> MSYSAYFAKAGFQFPAGLSALVAGIVALNVCTG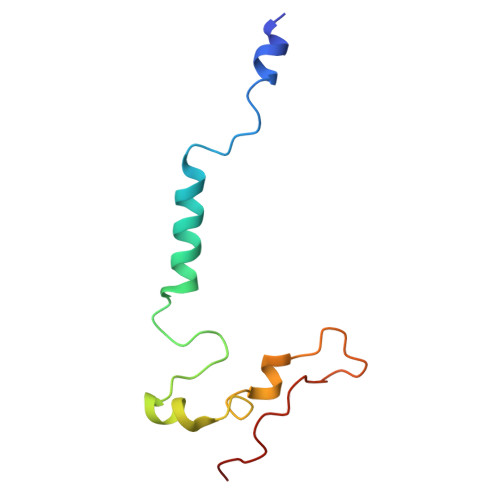RPTKGTKEISNAEYNATPIGYLQSPDQHPTAFPKVPGMKDVHGSPHHHH> MAKGEGAESGSAAGLLPTSILQASERPVQVKKEPKKKQQLSICNKLCYAVGGAPYQLTGCALGFFLHIYLLDVAKVEPLPASIILFVGRAWDAFTDPLVGFCISKSSWTRLGRLMPWIIFSTPLAIIAYFLIWFVPDFPSGTESSHGFLWYLLFYCLFETLVTCFHVPYSALTMFISTEQSERDSATAYRMTVEVLGTVIGTAIQGQIVGQAKAPCLQDQNGSVVVSEVANRTQSTASLKDTQNAYLLAAGIIASIYVLCAFILILGVREQRELYESQQAESMPFFQGLRLVMGHGPYVKLIAGFLFTSLAFMLVEGNFALFCTYTLDFRNEFQNLLLAIMLSATFTIPIWQWFLTRFGKKTAVYIGIS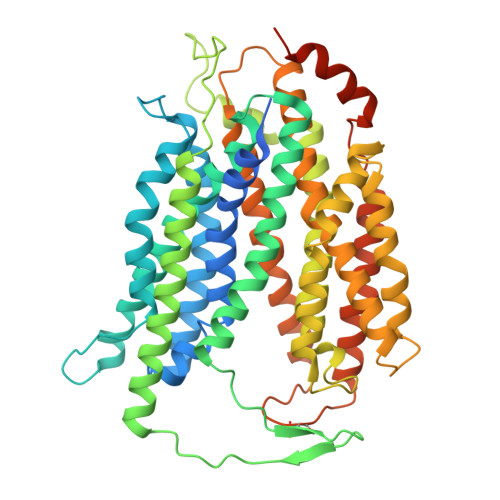SAVPFLILVALMERNLIVTYVVAVAAGVSVAAAFLLPWSMLPDVIDDFHLKHPHSPGTEPIFFSFYVFFTKFASGVSLGVSTLSLDFANYQRQGCSQPEQVKFTLKMLVTMAPIILILLGLLLFKLYPIDEEKRRQNKKALQALREEASSSGCSDTDSTELASIL>[2x]MPQDVDFHIPLPGRQSPDHARAEAEQLAWPRSLGLIRSDAAAERHLRGGYADLASRFYPHATGADLDLGVDLMSWFFLFDDLFDGPRGENPEDTKQLTDQVAAA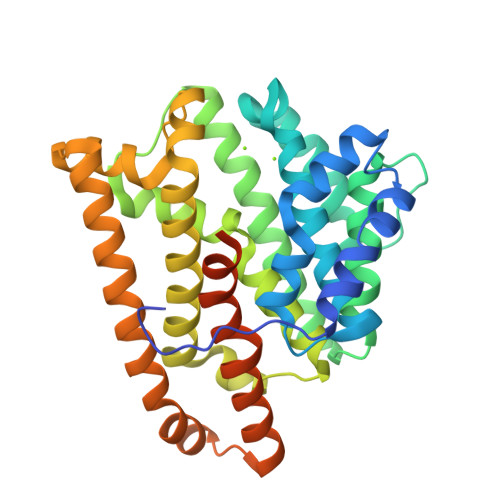LDGPLPDTAPPIAHGFADIWRRTCEGMTPAWCARSARHWRNYFDGYVDEAESRFWNAPCDSAAQYLAMRRHTIGVQPTVDLAERAGRFEVPHRVFDSAVMSAMLQIAVDVNLLLNDIASLEKEEARGEQNNMVMILRREHGWSKSRSVSHMQNEVRARLEQYLLLESCLPKVGEIYQLDTAEREALERYRTDAVRTVIRGSYDWHRSSGRYDAEFALAAGAQGYLEELGSSAH>GAMDPDLEATLRAIVHSATSLVDARYGAMAVHDRQHRVLHFVYEGIDEETVRRIGHLPKGLGVIGLLIEDPKPLRLDDVSAHPASIGFPPYHPPMRTFLGVPVRVRDESFGTLYLTDKTNG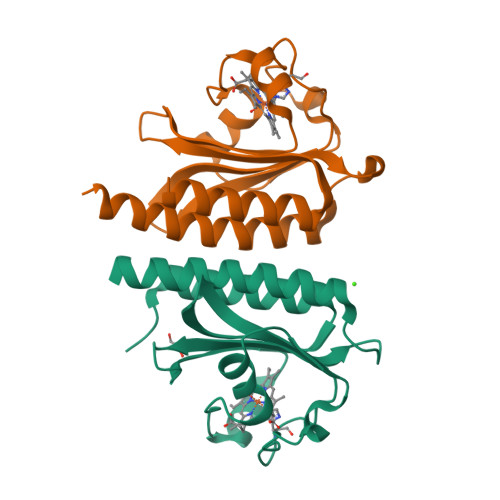QPFSDDDEVLVQALAAAAGIAVANARLYQQAK[2x]> QSMIPDFMSFTSHIDELYESAKKQSGGKVADYIPQLAKFSPDLWGVSVCTVDGQRHSTGDTKVPFCLQSCVKPLKYAIAVNDLGTEYVHRYVGKEPSGLRFNKLFLNEDDKPHNPMVNAGAIVVTSLIKQGVNNAEKFDYVMQFLNKMAGNEYVGFSNATFQSERESGDRNFAIGYYLKEKKCFPEGTDMVGILDFYFQLCSIEVTCESASVMAATLANGGFCPITGERVLSPEAVRNTLSLMHSCGMYDFSGQFAFHVGLP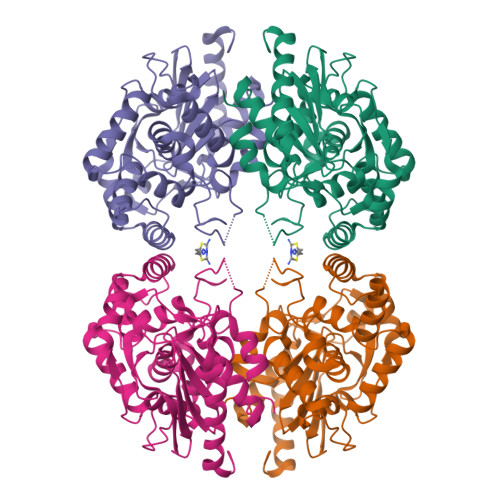AKSGVAGGILLVVPNVMGMMCWSPPLDKMGNSVKGIHFCHDLVSLCNFHNYDNL>MDIKINDITLGNNSPFVLFGGINVLESLDSTLQTCAHYVEVTRKLGIPYIFKASFDKANRSSIHSYRGVGLEEGLKIFEKVKAEFGI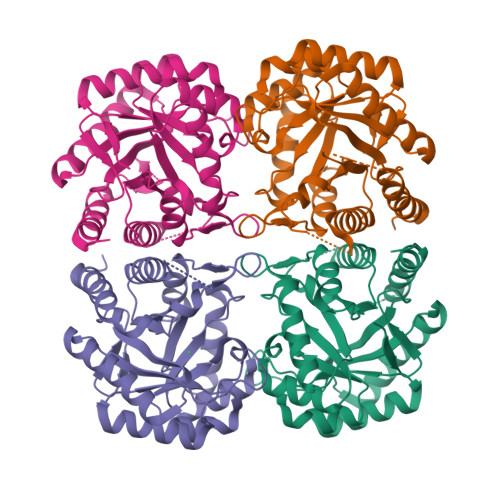PVITDVHEPHQCQPVAEVCDVIQLPAALARQTDLVVAMAKTGNVVNIKKPQFLSPSQMKNIVEKFHEAGNGKLILCERGSSFGYDNLVVDMLGFGVMKQTCGNLPVIFDVTHSLQTRDAGSAASGGRRAQALDLALAGMATRLAGLFLESHPDPKLAKCDGPSALPLHLLEDFLIRIKALDDLIKSQPILTIE[4x]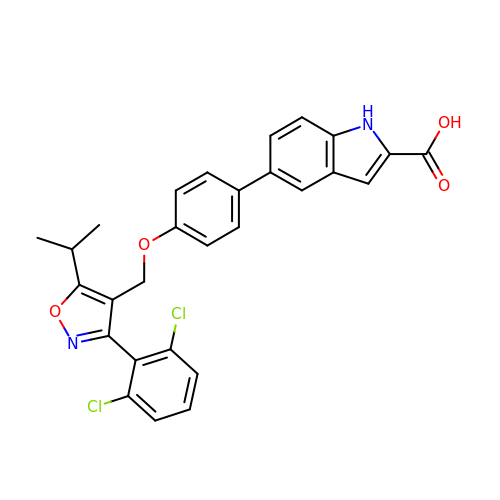5-(4-{[3-(2,6-dichlorophenyl)-5-(propan-2-yl)-1,2-oxazol-4-yl]methoxy}phenyl)-1H-indole-2-carboxylic acid | C28 H22 Cl2 N2 O4 | RYEIPXVNZXWZFN-UHFFFAOYSA-N>[2x]MAKKKKKKSFNTTRPTDPPVYPVTVPFLGHIVQFGKNPLEFMQRCKRDLKSGVFTISIGGQRVTIVGDPHEHSRFFSPRNEILSPREVYTIMTPVFGEGVAYAAPYPRMREQLNFLAEELTIAKFQNFVPAIQHEVRKFMAENWKEDEGVINLLEDCGAMIINTACQCLFGEDLRKRLNARHFAQLLSKMESSLIPAAVFMPWLLRLPLPQSARCREARAELQKILGEIIVAREKEEASKDNNTSDLLGGLLKAVYRDGTRMSLHEVCGMIVAAMFAGQHTSTITTSWSMLHLMHPKNKKWLDKLHKEIDEFPAQLNYDNVMDEMPFAERCVRESIRRDPPLLMVMRMVKAEVKVGSYVVPKGDIIACSPLLSHHDEEAFPNPRLWDPERDEKVDGAFIGFGAGVHKCIGQKFALLQVKTILATAFREYDFQLLRDEVPDPDYHTMVVGPTLNQCLVKYTRKKKLPSHHHHHH

Trypansoma cruzi, the protozoan agent of Chagas Disease, is closely related to two other major global pathogens, Leishmania spp., responsible for leishmaniasis, and Trypansoma brucei, the causative agent of African Sleeping Sickness. Both T. cruzi and Leishmania parasites have an essential requirement for ergosterol, and are thus vulnerable to inhibitors of sterol 14α-demethylase (CYP51), which catalyzes the conversion of lanosterol to ergosterol. Here we report the crystal structures for the CYP51 target in T. cruzi (CYP51Tc) (resolutions 2.35 Å and 2.27 Å) and that of the closely related CYP51 ortholog from Trypanosoma brucei (CYP51Tb) (resolutions 2.7 Å and 2.6 Å), each bound to an anti-fungal triazole drug, either fluconazole or posaconazole. Nevertheless, CYP51Tc and CYP51Tb do share 83% sequence identity, a fact which has been crucial for successfully determining their crystal structures and makes it possible to extrapolate structural features learned from one enzyme toward the other.

Although largely a backbone trace at 3.2 Å resolution, this structure served as a search model for molecular replacement in determining the CYP51Tc–fluconazole structure at 2.35 Å, which was used as a search model against the 2.27 Å CYP51Tc–fluconazole data to reveal an alternative conformation of fluconazole bound in the active site. The two CYP51Tc–fluconazole structures reported here superimpose with r.m.s.d of 0.68 Å, revealing some conformational differences in the F-helix and the BC-loop, which may account for the distinct fluconazole binding modes and result in re-packing of protein molecules in the crystal lattice. As expected, fluconazole is bound in the active site by coordination to the heme iron via the aromatic nitrogen atom of a triazole ring and by multiple van der Waals and aromatic stacking interactions. The 2,4-difluorophenyl moiety is enclosed in the pocket formed by the heme macrocycle, the aromatic side chains of Y103, F110, Y116 (BC-loop) and F290 (I-helix), and aliphatic side chains M106, A287 and A291. Although fluconazole occupies the same pocket in both CYP51Tc structures, it adopts two conformations that differ by the 180° flipping of the 2,4-difluorophenyl moiety. A 2.6 Å H-bonding contact between the 2-fluoro substituent and the hydroxyl group of Y103 may help to stabilize orientation 2, which appears to be less sterically favorable than orientation. In orientation 1, the H-bond between the 2-fluoro substituent and Y103 is broken due to the 3.5 Å reorientation of Y103 toward M360 resulting in the 2.7 Å H-bond to its amide nitrogen and in the flipping of the 2,4-difluorophenyl ring into a sterically more favorable orientation with the fluorinated edge facing away from the heme macrocycle. Perhaps both ring conformations co-exist in the CYP51Tc-fluconazole complex, possibly correlated with the conformation of the BC-loop which affects H-bonding pattern of Y103.The Picornaviridae family of single-stranded, positive-sense, non-enveloped RNA viruses includes several pathogens of concern such as enterovirus-D68 (EV68). The 3C protease cleaves eight sites within the viral polyprotein, with a preference for a glutamine–glycine (QG) motif at the P1/P1′ positions, a preference distinct from host cysteine proteases. Among strains of EV68, the amino acid sequences of 3C protease and its cleavage sites are highly conserved. We have determined and analyzed three high-resolution inhibitor-bound crystal structures of EV68-3C protease, which revealed possible sites of resistance mutations, a key structural water molecule conserved during ligand binding, and the conformational flexibility of the catalytic histidine H40.

Rupintrivir, AG7404, GC-376, and PF-00835231 showed inhibition against EV68-3C protease, while there was no observable inhibition with nirmatrelvir or ensitrelvir in this assay. We performed extensive co-crystallization trials with the 3C inhibitors that showed activity against EV68-3C in the enzymatic assays and achieved diffraction-quality crystals with rupintrivir, AG7404, and GC-376. The resulting structures are all the same space group (P3 21 1), had a clearly defined electron density for the entire inhibitor, and diffracted to sub 2 Å, facilitating direct comparison. GC-376, a smaller inhibitor, formed similar hydrogen bonds, with several residues found in all three inhibitors. Across all three structures, interactions between the inhibitor and Thr142, His161, Val162, and Gly164 were conserved. Within the S1 pocket, the g-lactam ring extended beyond the substrate envelope into the solvent. Based on this observation, mutations at Gly166 or Ala144 could introduce a steric bulk, blocking the protruding P1 moieties and decreasing the inhibitor’s ability to bind without impacting substrate binding. From these data, we predict that GC-376 would have a higher barrier to resistance compared to rupintrivir or AG7404.

> GPGFDFAQAIMKKNTVVARTEKGEFTMLGVHDRVAVIPTHASVGETIYINDVETKVLDACALRDLTDTNLEITIVKLDRNQKFRDIRHFLPRYEDDYNDAVLSVHTSKFPNMYIPVGQVTNYGFLNLGGTPTHRILMYNFPTRAGQCGGVVTTTGKVIGIHVGGNGAQGFAAMLLHSYFTDTAKHHHHHH>MTKKVAIILANEFEDIDYSSPKEALENAGFNTVVIGDTANSEVVGKHGEKVTVDVGIAEAKPEDYDALLIPGGFSPDHLRGDTEGRYGTFAKYFTKNDVPTFAICHGPQILIDTDDL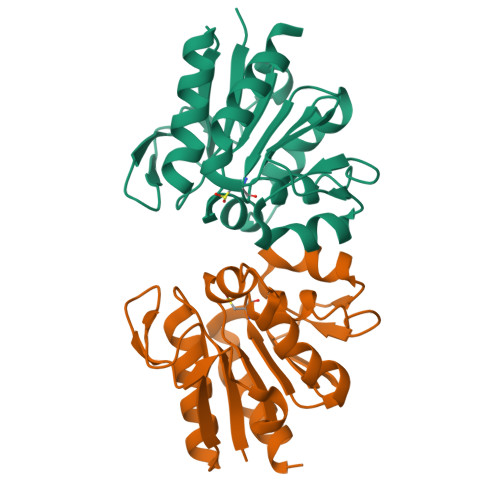KGRTLTAVLNVRKDLSNAGAHVVDESVVVDNNIVTSRVPDDLDDFNREIVKQLQLEHHHHHH[2x]>[2x]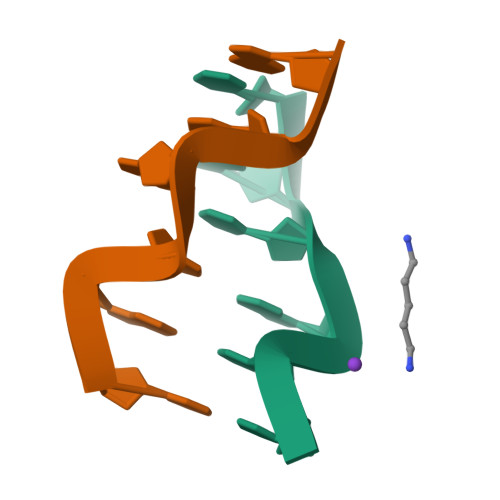CGCGCG>MGFKEYYRVFPTYTDINSQEYRSRIETLEPLLMKYMKKRGKVLDLACGVGGFSFLLEDYGFEVVGVDISEDMIRKAREYAKSRESNVEFIVGDARKLSFEDKTFDYVIFIDSIVHFEPLELNQVFKEVRRVLKPSGKFIMYFTDLRELLPRLKESLVVGQKYWISKVIPDQEERTVVIEFKSEQDSFRVRFNVWGKTGVELLAKLYFTKEAEEKVGNYSYL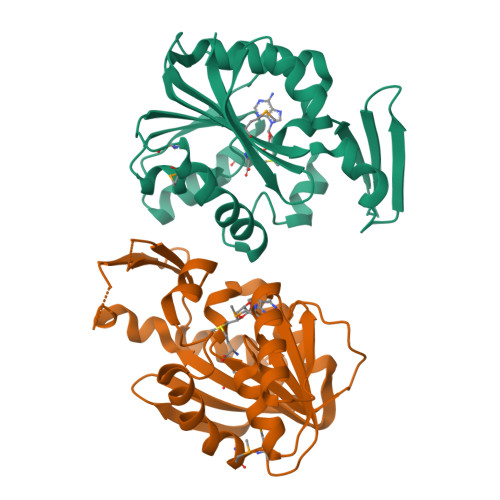TVYNPK[2x]>[4x]GNIESIENLQGIRALQQQAPQL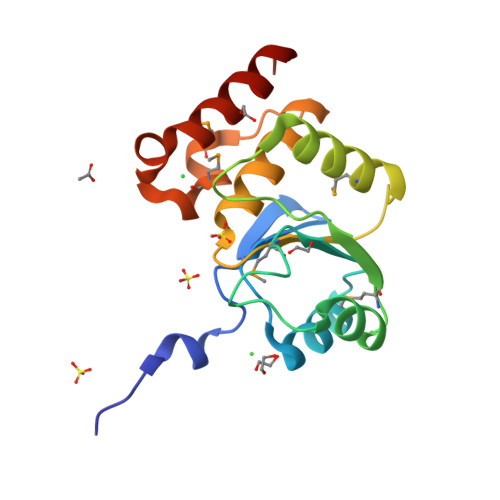LSSGLPNEQQFSLLKQAGVDVVINLMPDSSKDAHPDEGKLVTQAGMDYVYIPVDWQNPKVEDVEAFFAAMDQHKGKDVLVHCLANYRASAFAYLYQLKQGQNPNMAQTMTPWNDELAIYPKWQALLTEVSAKYGH> MTLVHNWHLGRRMEYPYFESRPKHQFAAVFNINRCIACQTCT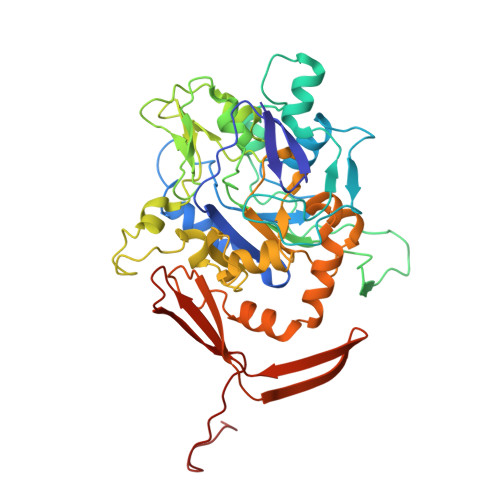MACKSTWTFNKGQEFMWWNNVETKPYGGFPQSWDVKTLKLIDSPDNIWYTDDKDKETSQYGTGAPYGTYEGDTIFEVAKKKNINQWAVGYIPEDKEWRSPNFGEDTAKSSNQPGEYSTLPEHSRWFFYLQRICNHCTYPGCLAACPRKAIYKRKEDGIVLIDQKRCRGYRKCVEQCPYKKPMYRGLTRVSEKCIACYPRIEGRDSLTDGRPMETRCMSACVGQIRLQGFLDDNPKNPITWLIRHQKIALPLYPQFGTEPNIYYIPPRWAPRAYLRQMFGPGVDEAIEKFMVPSRELLAVMSLFRMTQTIVYEYKIEEGPKVFETEIHGKKFTMYNDTVIGFGEDGKEVVRTTVEEPIHIRPDKHYNSI N-({(1S,2R)-2-[(S)-[(1R)-1-{[(BENZYLOXY)CARBONYL]AMINO}-2-PHENYLETHYL](HYDROXY)PHOSPHORYL]CYCLOPENTYL}CARBONYL)-L-TRYPTOPHAN | C33 H36 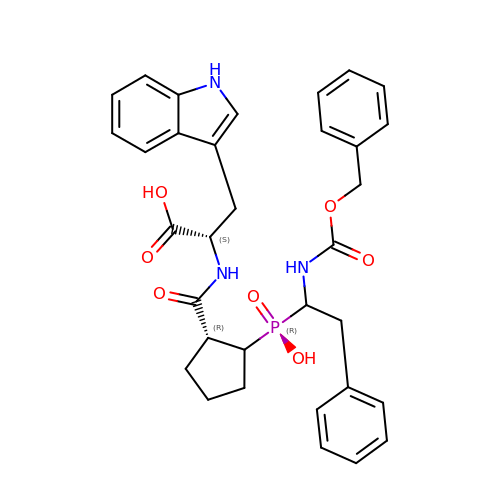N3 O7 P | IMPJIKIXNAGRCR-RRFVUZEHSA-N> SSKPDI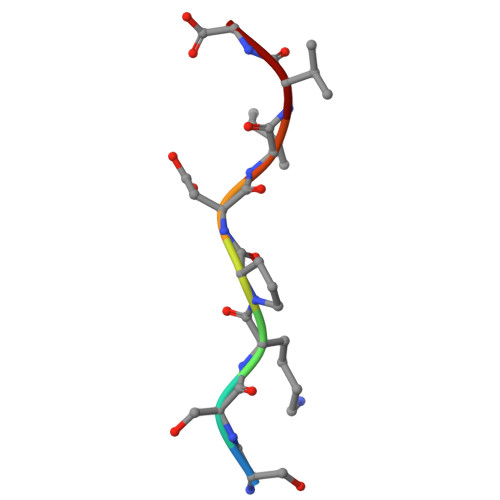VG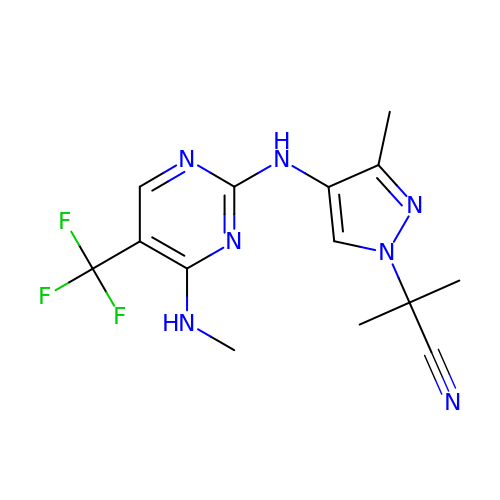2-methyl-2-(3-methyl-4-{[4-(methylamino)-5-(trifluoromethyl)pyrimidin-2-yl]amino}-1H-pyrazol-1-yl)propanenitrile | C14 H16 F3 N7 | ZPPUMAMZIMPJGP-UHFFFAOYSA-N> GCTGGATATA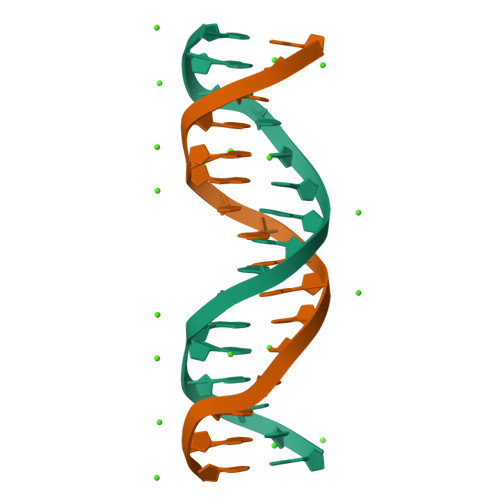TCCAGC> MMTMHKALTIAGSDSSGGAGIQADLKTFQELGVYGMSAITAIVAQNTLGHKGVYPLPLEAIEAQLDTVLEDIGVDALKTGMLATAEIIELVAEKIKEYNVKNVVVDPVMIAKGGDSLLHEEAAEALR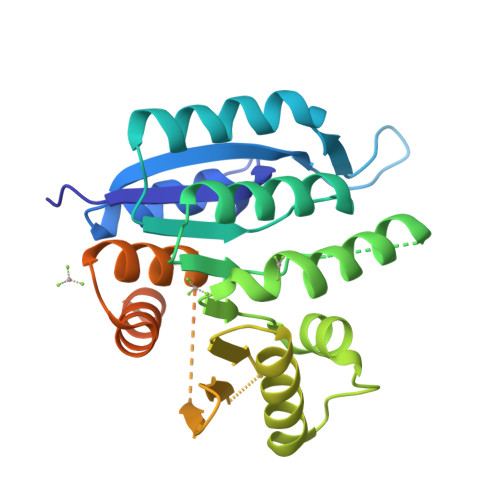EELIPLATVVTPNLPEAEVLSGMRIIKTVEDMKEAAKKIHEMGAKYVLVKGGHLEGDDEAVDVLFDGEEFEIFESERIDTKHTHGAGCTFSAAITAELAKGYSLKEAVKTAKEFITEAIRHSFPLGQGVGPTNHSAYREKEAKESETAEAPEAA>[2x]MDVVVRLPDVAVPGEAVQASARQAVIHLVDIAGITSSTPADYATKNLYLWNNETCDALSAPVADWNDVSTTPTGSDKYGPYWVIPLTKESGCINVIVRDGTNKLIDSDLRVSFSDFTDRTVSVIAGNSAVYDSRADAFRAAFGVALADAHWVDKTTLLWPGGENKPIVRLYYSHSSKVAADSNGEFSDKYVKLTPTTVSQQVSMRFPHLASYPAFKLPDDVNVDELLQGETVAIAAESDGILSSATQVQTAGVLDDTYAAAAEALSYGAQLTDSGVTFRVWAPTAQQVELVIYSADKKVIASHPMTRDSASGAWSWQGGSDLKGAFYRYAMTVYHPQSRKVEQYEVTDPYAHSLSTNSEYSQVVDLNDSALKPEGWDGLTMPHAQKTKADLAKMTIHESHIRDLSAWDQTVPAELRGKYLALTAQESNMVQHLKQLSASGVTHIELLPVFDLATVNEFSDKVADIQQPFSRLCEVNSAVKSSEFAGYCDSGSTVEEVLTQLKQNDSKDNPQVQALNTLVAQTDSYNWGYDPFHYTVPEGSYATDPEGTARIKEFRTMIQAIKQDLGMNVIMDV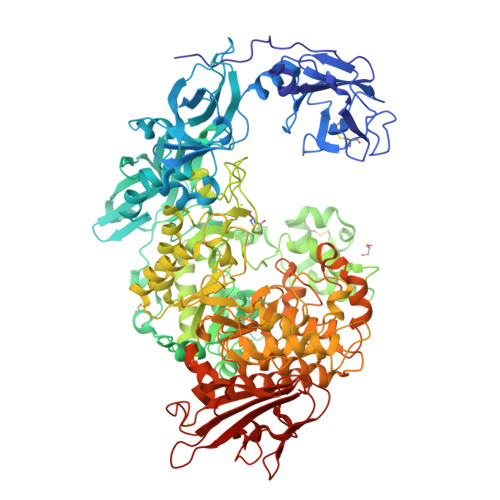VYNHTNAAGPTDRTSVLDKIVPWYYQRLNETTGSVESATCCSDSAPEHRMFAKLIADSLAVWTTDYKIDGFRFDLMLYHPKAQILSAWERIKALNPDIYFFGEGWDSNQSDRFEIASQINLKGTGIGTFSDRLRDAVRGGGPFDSGDALRQNQGVGSGAGVLPNELTTLSDDQARHLADLTRLGMAGNLADFVLIDKDGAVKRGSEIDYNGAPGGYAADPTEVVNYVSKHDNQTLWDMISYKAAQEADLDTRVRMQAVSLATVMLGQGIAFDQQGSELLRSKSFTRDSYDSGDWFNRVDYSLQDNNYNVGMPRSSDDGSNYDIIARVKDAVATPGETELKQMTAFYQELTALRKSSPLFTLGDGATVMKRVDFRNTGADQQTGLLVMTIDDGMQAGASLDSRVDGIVVAINAAPESRTLQDFAGTSLQLSAIQQAAGDRSLASGVQVAADGSVTLPAWSVAVLELPQGESQGAGLPVSSK>MRIPLVGKDSIESKDIGFTLIHEHLRAFSEAVRQQWPHLYNEDEEFRNAVNEVKRAMQFGVKTIVDPTVMGLGRDIRFMEKVVKATGINLVAGTGIWIYIDLPFYFLNRSIDEIADLFIHDIKEGIQGTLNKAGFVKIAADEPGITKDVEKVIRAAAIANKETKVPIITHSNAHNNTGLEQQRILTEEGVDPGKILIGHLGDTDNIDYIKKIADKGSFIGLDRYGLDMFLPVDKRNETTLRLIKDGYSDKIMISHDYCCTIDWGTAKPEYKPKLAPRWSITLIFEDTIPFLKRNGVNEE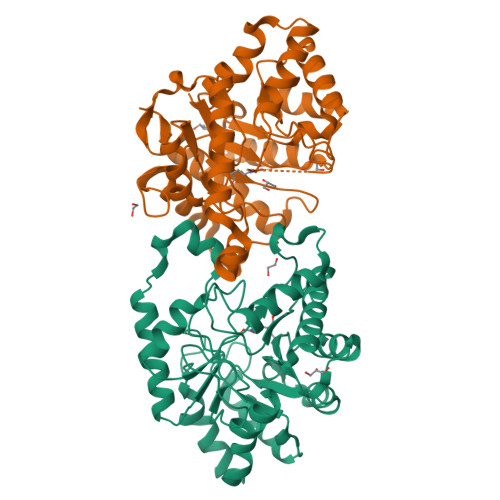VIATIFKENPKKFFS[4x]> MTGGMKPPARKPRILNSDGSSNITRLGLEKRGWLDDHYHDLLTVSWPVFITLITGLYLVTNALFALAYLASGDVIENARPGSFTDAFFFSVQTMATIGYGKLIPIGPLANTLVTLEALCGMLGLAVAASLIYARFTRPTAGVLFSSRMVISDFEGKPTLMMRLANLRIEQIIEADVHLVLVRSEISQEGMVFRRFHDLTLTRSRSPIFSLSWTVMHPIDHHSPIYGETDETLRNSHSEFLVLFTGHHEAFAQNVHARHAYSSDEIIWGGHFVDVFTTLPDGRRALDLGKFHEIAQHHHHHH

We have utilised the prokaryotic Kir channel KirBac3.1 to determine whether the acyl tails of bound lipids, protruding into the conduction pathway through fenestrations just below the selectivity filter, might represent key gating elements. In KirBac3.1, the four Leu124 residues form a steric cluster physically occluding the conduction pathway, separating the cavity into upper and lower vestibules, while Tyr132 (at the inner helix bundle) forms a non-occlusive hourglass-shaped portal between lower vestibule and cytosol. Here we present evidence that in Kir channels, a limiting barrier to permeation within the conduction pathway is formed by a collar of branched aliphatic side chains. We show that acyl tails of tightly bound lipids occupying conserved fenestrations into the pore engage individual side chains of the collar, drawing them away from the central conduction pathway and allowing ions to pass.

The mutation was made on a background in which two native cysteines were mutated to serine (C71S-C262S; SCS) and thus we also determined a structure of the KirBac3.1-SCS background crystallised under the same conditions. To cross-validate this experimentally, we mimicked isolated lipid tails using alkyl-methylthiosulfonate (alkyl-MTS) reagents, derivatising a native cysteine residue (Cys119) located near the midpoint of the bilayer at the outer opening to the fenestration on an otherwise cysteine-less background (SCS); the same background as used for L124M. All crystal structures of native KirBac3.1 show the conduction pathway is occluded by a Leu124 cluster, indicative of a favoured low-energy state. In every instance, we observed extended fatty acyl chains of lipids occupying fenestrations near the midpoint of the lipid bilayer, a phenomenon also observed in crystal structures.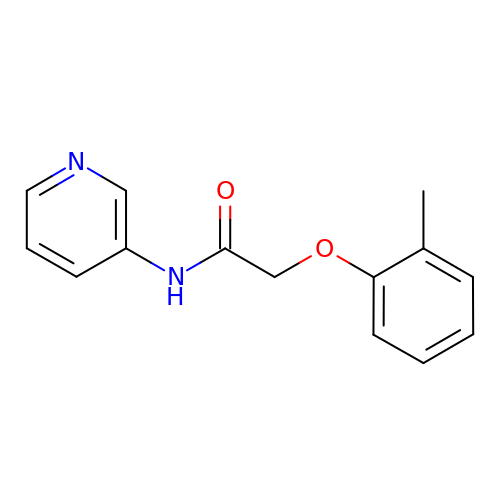2-(2-methylphenoxy)-~{N}-pyridin-3-yl-ethanamide | C14 H14 N2 O2 | MUOTYWWZYLNCGX-UHFFFAOYSA-N>GAMAQLAAPLKVGAIYTIGPYLFPHLIPQLHRVAPQMPLYIEENFTHILRDKLRTGELDAIIIALPFQEADVLTKPLFDEPFYVLMPADHPWTAKASIDSELLNDKSLLLLGEGHDFRDQVLEACPTVRKGDENKHTTVESSSLETIRHMVASGLGVSVLPFSAVDSHHYAPGVIEVRP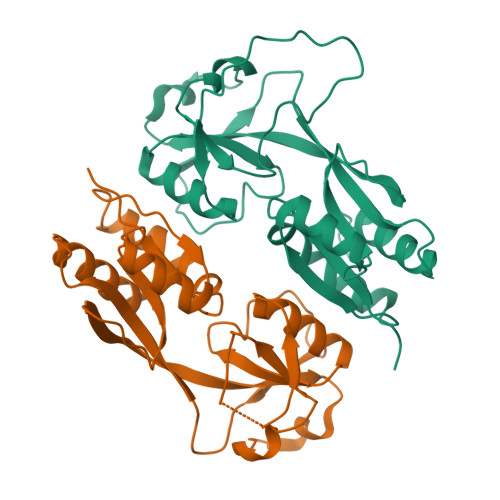FSAPVPFRTVAIAWRASFPRPRAIEVLADSIRLCSVARPQTQEQPQIA[4x]> MVSSKKFNQVDKGRGMISENYIEPAFLLPDLIEIQRSSFRWFLEEGLIEELNSFSPITDYTGKLELHFLGHNYKLKEPKYSVEEAKRRDSTYAVQMYVPTRLLNKETGDIKEQEVFIGDLPLMTDRGTFI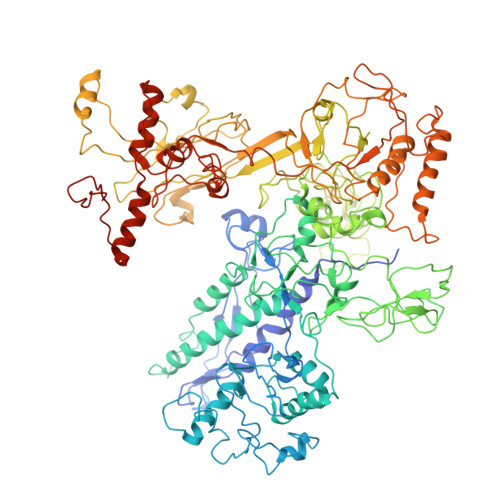INGAERVIVNQIVRSPGVYYKSEIDKNGRRTYSASLIPNRGAWLKFETDRNDLVWVRIDKTRKLSAQVLLKALGLSDNEIFDALRHPEYFQKTIEKEGQFSEEEALMELYRKLRPGEPPTVLGGQQLLDSRFFDPKRYDLGRVGRYKLNKKLRLSVPDTVRVLTSGDILAAVDYLINLEYDIGSIDDIDHLGNRRVRSVGELLQNQVRVGLNRLERIIRERMTVSDAEVLTPASLVNPKPLVAAIKEFFGSSQLSQFMDQTNPLAELTHKRRLSALGPGGLTRERAGFAVRDIHPSHYGRICPIETPEGPNAGLIGSLATHARVNQYGFLETPFRPVENGRVRFDQPAAYMTADEEDDLRVAPGDIPVDENGYIIGPQVPVRYRQEFSTTTPEQVDYVAVSPVQIVSVATSMIPFLEHDDANRALMGSNMQRQAVPLLKPERPLVGTGLEAQGARDSGMVIVSRTDGDVVYVDATEIRVRVSGQLPTASGKSTDNGQLTSQKGQEIRYTVSKYQRSNQDTCLNQKPLVRIGERVVAGQVLADGSSTEGGELALGQNIVVAYMPWEGYNYEDAILISERLVQDDIYTSIHIEKYEIEARQTKLGPEEITREIPNVGEDALRQLDEQGIIRIGAWVEAGDILVGKVTPKGESDQPPEEKLLRAIFGEKARDVRDNSLRVPNGEKGRVVDVRLFTREQGDELPPGANMVVRVYVAQKRKIQVGDKMAGRHGNKGIISRILPIEDMPYLPDGSPVDIVLNPLGVPSRMNVGQVFECLLGWAGHTLGVRFKITPFDEMYGEESSRRIVHGKLQEARDETGKDWVYNPDDPGKIMVYDGRTGEAFDRPVTIGVAYMLKLVHLVDDKIHARSTGPYSLVTQQPLGGKAQQGGQRFGEMEVWALEAFGAAYTLQELLTVKSDDMQGRNEALNAIVKGKAIPRPGTPESFKVLMRELQSLGLDIAVHKVETQADGSSLDVEVDLMADQLARRTPPRPTYESLSRESLDDDE> MQKLTVGLIGNPNSGKTTLFNQLTGARQRVGNWAGVTVERKEGIFATTDHQVTLVDLPGTYSLTTISSQTSLDEQIACHYILSGDADMLINVVDASNLERNLYLTLQLLELGIPCVVALNMLDIAEKQQVRIDIDALAARLGCPVIPLVSTRGRGIEALKIALDRHQANSDLELVHYPQPLLREADLLAQQMSAQIPPRQRRWLGLQMLEGDIYSRAYAGDAADKLDIALANLS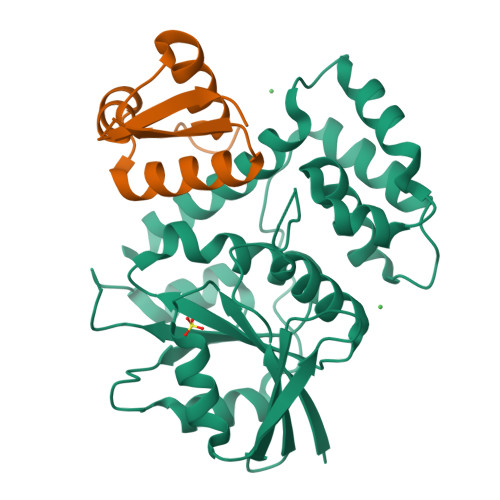DEIDDPALHIADARYQTIAAICDAVSNTLTAEP;> PLGSMASLMEVRDMLALQGRMEAKQLSARLQTPQPLIDAMLERMEAMGKVVRISETSEGCLSGSCKSCPEGKAACRQEWWALRL>[15x]VTPGAILVTHPLESYYNQFLDGLPTSELEELEIEFVAMCIGFPRSQNNFVNALLDLSTIEVYTIRTSVKEILRLDKLNKESIENRQVTKVEDITMNMNYIGDIKDELVTEVKKLARILKLPVLDNLYVSYDDVEGRIGANGLLEPLNRGSGFGSYLTGYTVR;>MRRLKGTIRHLDDQPWINVSLFLTLINGTFNSANQYPIDTKHAKTDQNGEFVFNVVPNVGIDQSYYILTTPDNKKHSFTVPDGTSDIEFSVVREAGIIATDPEYTNVLNYLEDYIDDAIANIQASSVIAEIFTCGQTISALKALRFDSSTGKVFYASSSDATHLNKCVGVSSQSGVLNDNIQVVTSGYLSDQSWNWTIGSPIFFDSGGTLTHTPGSSYYQVIGIPVTTNKVLISVEQPIKL[15x]

A-1(L) is a Myoviridae cyanophage isolated in 1970s9 that specifically infects the model cyanobacterium Anabaena sp. PCC 7120. Using cryo-electron microscopy (cryo-EM), we solved the structure of A-1(L) tail machine, which consists of three parts: a 205-Å-long neck, a 1045-Å-long contractile tail with a complicated baseplate, and six pairs of tail fibers. The dodecameric gp2 portal, the pentadecameric gp5 and the hexameric gp7 sequentially constitute the neck of A-1(L), to which five neck fibers are attached. The long and contractile tail of A-1(L) contains 24 rings of gp10 hexamers that form the tube, surrounded by the sheath of 24 helically stacked gp9 hexamers.

After multiple rounds of attempt, the structures of gp5 and gp5-gp82N complex were finally solved by imposing C15 and C5 symmetry, respectively. Structural analysis showed that the neck/gp5 consists of 15 subunits of different fold compared to those previously solved counterparts; however, it possesses a same 15-fold symmetry as the recently reported collar sheath protein of Agrobacterium phage Milano that crosslinks the tail sheath to the neck. At the 5-fold vertex of A-1(L) capsid, the 12-fold portal/gp2 dodecamer, the 15-fold neck/gp5 pentadecamer, and the 6-fold neck/gp7 hexamer are sequentially interlocked to form a symmetry-mismatched neck. Moreover, the trimeric N-terminal domain of gp82 (gp82N, residues Met1-Ser125) of each neck fiber attaches to the gp5, whereas the C-terminal domain of gp82 (gp82C, residues Ser126-Leu241) and beyond of the flexible neck fiber could not be modeled due to the poor EM density. In detail, the ring formed by Loopα4-α5 (residues Ile83-Tyr99) of 15 gp5 subunits is hooked by six long α1 helices (residues Met1-Leu25) at the N-terminus of gp7, whereas Loopα1-α2 (residues Leu20-Glu30) of three gp5 subunits tightly interact with the Loopβ5-β6 (residues Thr70-Lys75) of trimeric gp82N. Each neck fiber comprises a trimeric gp82 with the N-terminal domain clearly modeled, followed by the highly flexible components gp80 and gp81. The results showed that gp82 indeed possesses two separate domains gp82N and gp82C, which are attached to gp5 and extended outwards, respectively. A-1(L) possesses five neck fibers with gp82N tightly attached to the pentadecameric neck/gp5, representing a neck and neck fiber of distinct symmetry. Notably, the neck fiber gp82N adopts a fold similar to the previously reported component of bacterial pilus. Notably, the interface between the 12-fold gp2 and the 15-fold gp5 possesses a rather poor density map, indicating that the relative orientations between symmetry-mismatched gp2 and gp5 vary in A-1(L) particles. Moreover, we found that the purified gp82-gp81 and gp81-gp80 complexes could also form a bead-chain-like structure, which suggested that the neck fiber is independently self-assembled in prior of being hooked to the neck via gp82N.> SETQANSTTDALNVLLIIVDDLRPSLGCYGDKLVRSPNIDQLASHSLLFQNAFAQQAVAAPSRVSFLTGRRPDTTRLYDFNSYWRVHAGN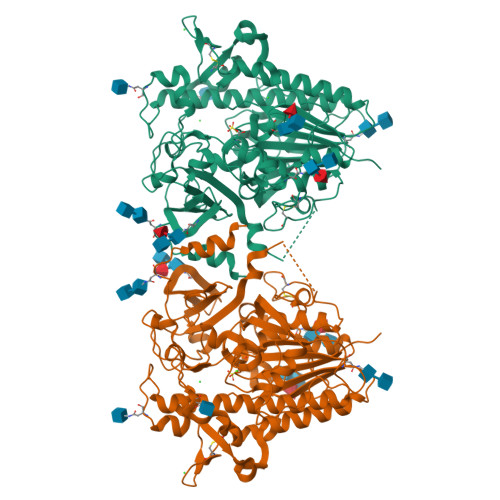FSTIPQYFKENGYVTMSVGKVFHPGISSNHTDDSPYSWSFPPYHPSSEKYENTKTCRGPDGELHANLLCPVDVLDVPEGTLPDKQSTEQAIQLLEKMKTSASPFFLAVGYHKPHIPFRYPKEFQKLYPLENITLAPDPEVPDGLPPVAYNPWMDIRQREDVQALNISVPYGPIPVDFQRKIRQSYFASVSYLDTQVGRLLSALDDLQLANSTIIAFTSDHGWALGEHGEWAKYSNFDVATHVPLIFYVPGRTASLPEAGEKLFPYLDPFDSASQLMEPGRQSMDLVELVSLFPTLAGLAGLQVPPRCPVPSFHVELCREGKNLLKHFRFRDLEEDPYLPGNPRELIAYSQYPRPSDIPQWNSDKPSLKDIKIMGYSIRTIDYRYTVWVGFNPDEFLANFSDIHAGELYFVDSDPLQDHNMYNDSQGGDLFQLLMP> MENLVRLRDSFAWVQQTNKALLAISAIQQAVLE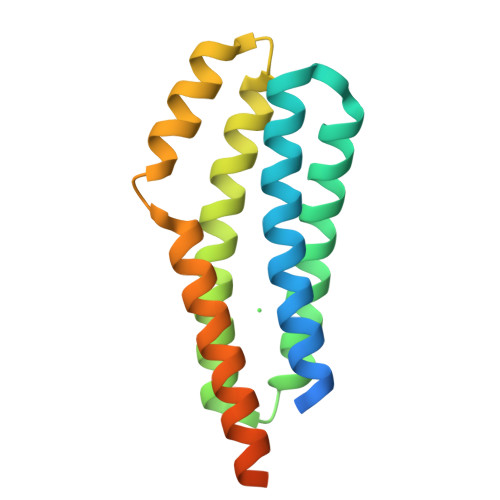AETSERGFLLTGIETYRDSYIRARDALAARLDGLRAVLADNPEQIAHIDELRLLTDMRMAQLGRVVELGPERMREALDILEQARVDRLTERIETSLSVLTRAEQALLIQRLSKHDRESLAAALLEHHHHHH> MNQIDLNVTCRYAGVFHVEKNGRYSISRTEAADLCQAFNSTLPTMDQMKLALS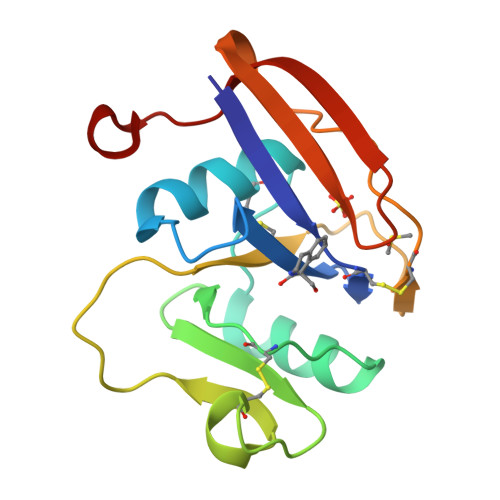KGFETCRYGFIEGNVVIPRIHPNAICAANHTGVYILVTSNTSHYDTYCFNASAPPEEDCTSVTDLPNSFDGPVTITIVNRDGTRYSKKGEYRTHQEDI[1-[(2~{S},3~{S},4~{R},5~{S},6~{R})-2-[(1~{S},2~{S},4~{S},5~{S})-2-(2-chloroethyloxy)-4,5-bis[[4-(hydroxymethyl)phenyl]methylcarbamoyl]cyclohexyl]oxy-6-(hydroxymethyl)-4,5-bis(oxidanyl)oxan-3-yl]-1,2,3-triazol-4-yl]methylazanium 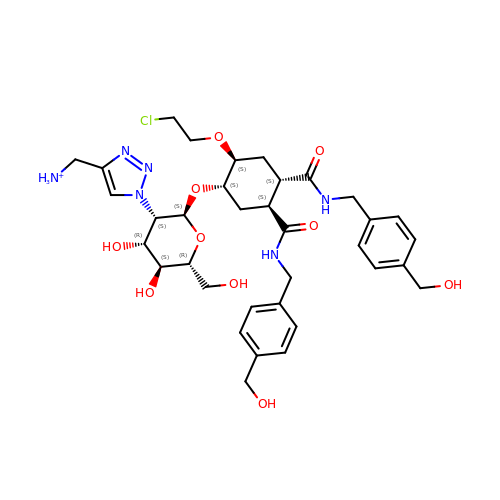| C35 H48 Cl N6 O10 | BYGZQFCUFRSCML-RWSQSUCKSA-O> MSSGAVGRGSFHSVVAGANPRRIPTYYNSAYEL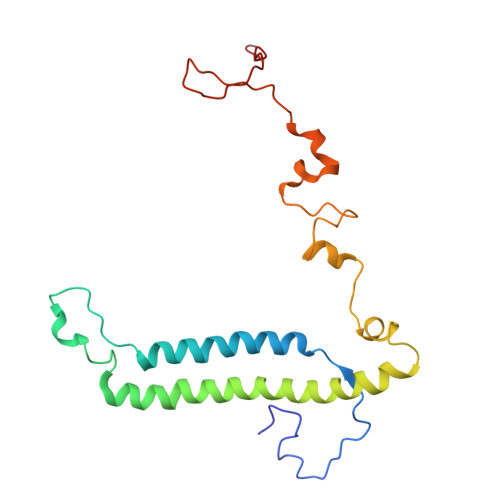IQLHRAHREVTRNFLVRDKVFDNKFPGCSLANGLFKMVPNKRGNFHTRELTESIRHRTIWGQRIQQQRTINAAILEDATKVLSPAQMEDRFSYRTPDAAAYFSPQEYTAANNWPNYWQHPTEKHVVPKPRWRREPELGGITRVRDAVATPIADY>[6x]MSLDVRQSIHSAHAKTLDTQGLRNEFLVEKVFVADEYTMVYSHIDRIIVGGIMPITKTVSVGGEVGKQLGVSYFLERRELGVINIGGAGTITVDGQCYEIGHRDALYVGKGAKEVVFASIDTGTPAKFYYNCAPAHTTYPTKKVTPDEVSPVTLGDNLTSNRRTINKYFVPDVLETCQLSMGLTELAPGNLWNTMPCHTHERRMEVYFYFNMDDDACVFH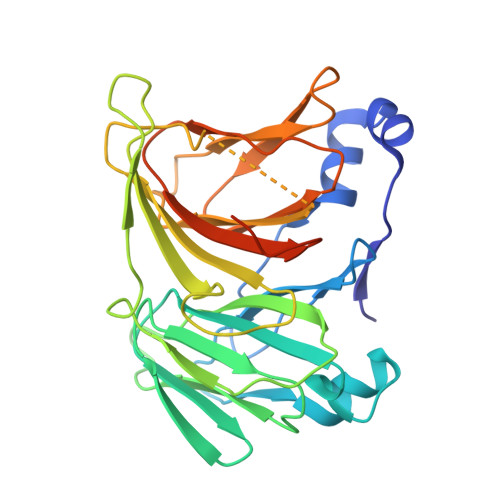MMGQPQETRHIVMHNEQAVISPSWSIHSGVGTKAYTFIWGMVGENQVFDDMDHVAVKDLREGHHHHHH>[2x]MAHHHHHHMSTDWIPISQ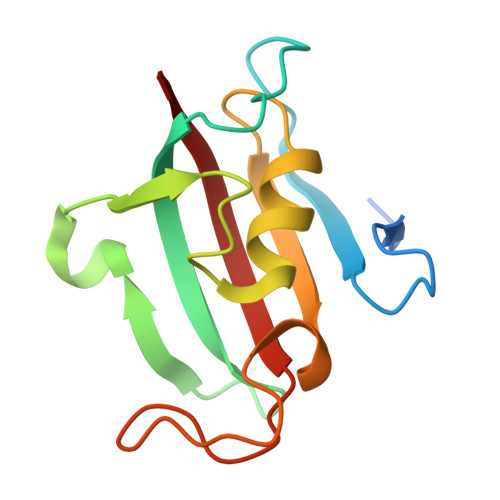DQRLKKKIITAGSSDEQPPIGSKVSVHYTGTLTSGKKFDSSLDRGQPFVFTLGKGEVIRGWDLGVKSMKKGEKSYFEIPSDYAYGNNAIPGLIPANSTLMFEIELLSWK Central to these functions, RAD52 promotes the annealing of complementary single-stranded DNA (ssDNA)8,9 and provides an alternative to BRCA2/RAD51-dependent homologous recombination repair. Instead, cryo-electron microscopy and biochemical analyses revealed that ssDNA annealing is driven by RAD52 open rings in association with replication protein-A (RPA). RPA associates with RAD52 at the site of ring opening with critical interactions occurring between the RPA-interacting domain of RAD52 and the winged helix domain of RPA2. Our studies provide structural snapshots throughout the annealing process and define the molecular mechanism of ssDNA annealing by the RAD52–RPA complex.

When visualized using cryo-EM, we found that the two species of full-length RAD52 represent open (RAD52-OR, peak 1) and closed (RAD52-CR, peak 2) ring forms. The 11-subunit closed rings exhibit features similar to the RAD52 NTD, whereas the RAD52 open rings have one or more subunits missing. The structures of RAD52-CR (2.9 Å) and RAD52-OR (3.2 Å) were determined using cryo-EM. The RAD52-OR structures contained a maximum of ten subunits, although open rings with fewer subunits were also observed. The structure of each subunit in the open ring was similar to that of the closed ring. As expected, the cryo-EM density around the site of ring opening was not as well resolved as other parts of the structure. Consistent with this, in addition to the ten-subunit open ring, our analysis of two-dimensional (2D) averages and three-dimensional (3D) classes indicated the presence of RAD52-OR structures with fewer subunits. The RAD52 open rings exhibited a high affinity (KD = 0.3 ± 0.1 nM) for 40-nucleotide-long ssDNA but not double-stranded DNA (dsDNA), as measured by fluorescence anisotropy. The RAD52-ORs annealed ssDNA in reactions stimulated by RPA, whereas the RAD52-CRs exhibited a reduced ability to promote annealing that was unaffected by the presence or absence of RPA. Importantly, RAD52 adopts open- and closed-ring configurations, such that the open rings represent the active form of the protein for SSA.

>[10x]MSGTEEAILGGRDSHPAAGGGSVLCFGQCQYTAEEYQAIQKALRQRLGPEYISSRMAGGGQKVCYIEGHRVINLANEMFGYNGWAHSITQQNVDFVDLNNGKFYVGVCAFVRVQLKDGSYHEDVGYGVSEGLKSKALSLEKARKEAVTDGLKRALRSFGNALGNCILDKDYLRSLNKLPRQLPLEVDLTKAKRQDLEPSVEEARYNSCRPNMALGHPQLQQVTSPSRPSHAVIPADQDCSSRSLSSSAVESEATHQRKLRQKQLQQQFRERMEKQQVRVSTPSAEKSEAAPPAPPVTHSTPVTVSEPLLEKDFLAGVTQELIKTLEDNSEKWAVTPDAGDGVVKPSSRADPAQTSDTLALNNQMVTQNRTPHSVCHQKPQAKSGSWDLQTYSADQRTTGNWESHRKSQDMKKRKYDPS>DKIPDFVVPGKCASVTRNKLWAEQTPNRNMYAGVWYQFALTNNPYQLIEKCVRNEYSFDGEQFVITSTGIAYDGNLLKRNGKLYPNPFGEPHLSIDYEMSFAAPLVILETDYSNYACLYSCIDYNFGYHSDFSFIFSR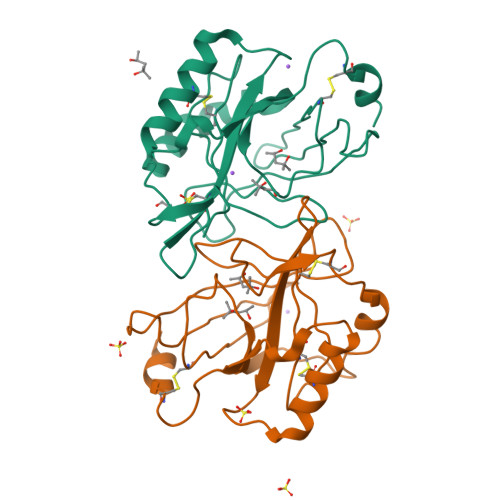SANLADKYVKKCEAAFKNINVDTTRFVKTVQGSSCPYDTQKTV[2x]> A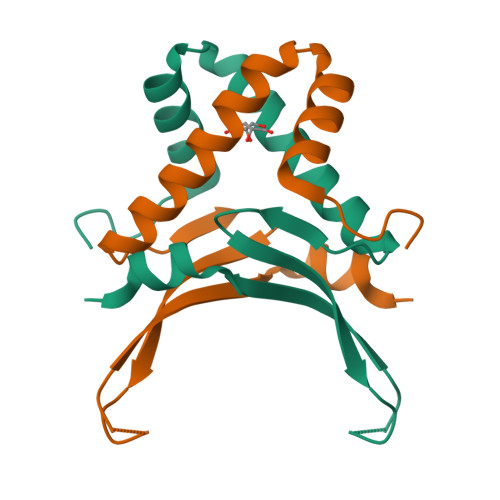AKKTVTKADLVDQVAQATGLKKKDVKAMVDALLAKVEEALANGSKVQLTGFGTFEVRKRKARTGVKPGTKEKIKIPATQYPAFKPGKALKDKVKK ADENOSINE 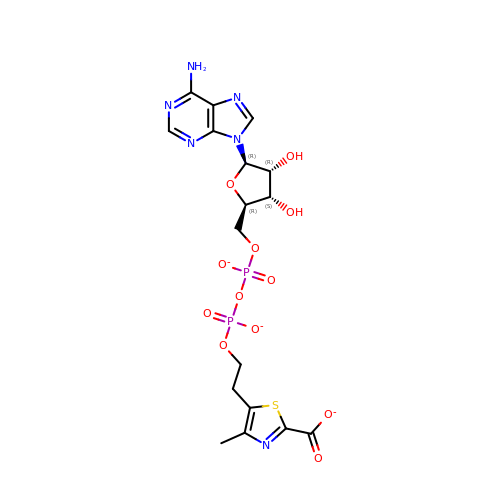DIPHOSPHATE 5-(BETA-ETHYL)-4-METHYL-THIAZOLE-2-CARBOXYLIC ACID | C17 H19 N6 O12 P2 S | VGXBGQACJQRWLV-LKGUXBDMSA-K> MPIIKEPIDFINKPESEAKEWGKEEEKRWFTKLNNLEEVAVNQLKNKEYKTKIDNFSTDILFSSLTAIEIMKEDENQNLFDVERIREALLKNTLDRDAIGYVNFTPKELGINFSIRDVELDRDISDETLDKVRQQIINQEYTKFSFISLGLNDNSINESVPVIVKTRVPTTFDYGVLNDKETVSLLLNQGFSIIPESAIITTIKGKDYILIEGSLSQELDFYNKGSEAWGAENYGDYISKLSHEQLGALEGYLHSDYKAINSYLRNNRVPNNDELNKKIELISSALSVKPIPQTLIAYRRVDGIPFDLPSDFSFDKKENGEIIADKQKLNEFIDKWTGKEIENLSFSSTSLKS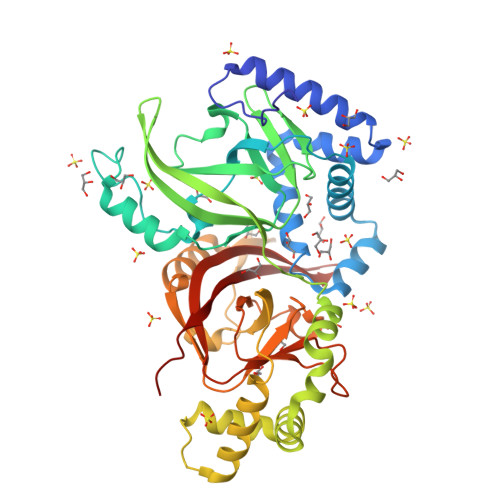TPSSFSKSRFIFRLRLSEGAIGAFIYGFSGFQDEQEILLNKNSTFKIFRITPITSIINRVTKMTQVVIDAEGIQNKEI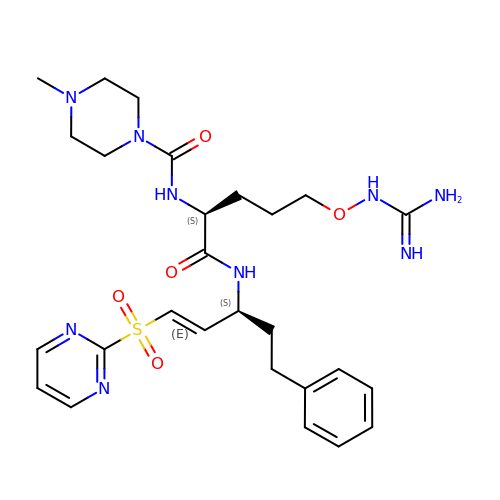N-[(2S)-5-(carbamimidamidooxy)-1-oxo-1-{[(1E,3S)-5-phenyl-1-(pyrimidin-2-ylsulfonyl)pent-1-en-3-yl]amino}pentan-2-yl]-4-methylpiperazine-1-carboxamide | C27 H39 N9 O5 S | FGWKPELIWHWYFZ-OBYRPWEKSA-N3-deoxy-3-[4-(thiophen-3-yl)-1H-1,2,3-triazol-1-yl]-beta-D-galactopyranosyl 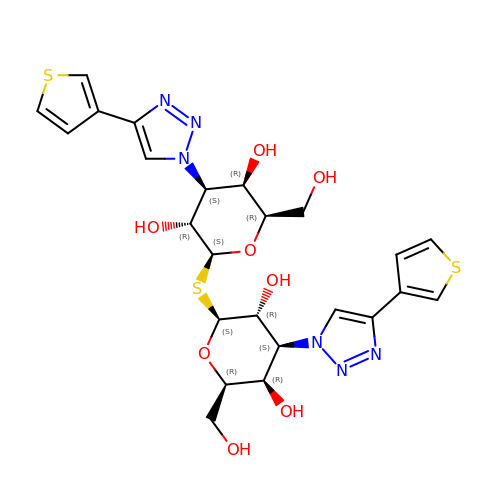3-deoxy-1-thio-3-[4-(thiophen-3-yl)-1H-1,2,3-triazol-1-yl]-beta-D-galactopyranoside | C24 H28 N6 O8 S3 | OYKAQKLJBYMZSV-VLLPDFJVSA-N>[2x]MTPNWSELVAAADPALVLPSGERRAEVAVPGPLRLDALLDLGEGHAVGVVRSADAARWTVPLVRDGAGGVRRSRPGDGTAEHLVAALARRGATPDAAFVLEAFTGAAPVTGERGIIVDQTNESVIVGECAVVKWAVRLPAEGEPGSPAAQRIAALARGGFTEMPRPWGLLTLAEGAQPVLLASVVAYLPGALDGWDWAVDDVRRLARGEL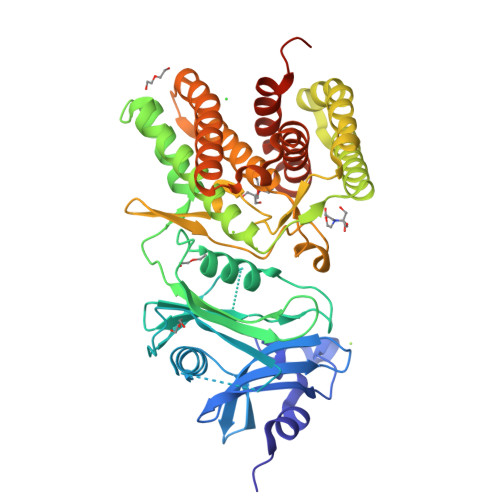TMDQALLPAAQLGTLTARMHAALAARGRTPATAADVAAWGVRMREELDEAVASVPGAEGERLKAWAPRIADVYAELDALAGTPLIDVHGDFHVGQILRADGRYAVVDFDGNPVLPADQRAARQPAALDVVGMTASLDHVGRVVVFRTPDVDPAPVRAWIAAAQRSFLDAYRTTLARLDADDLFDDRLLTPLRYAQEVREYLYAVRHLPHWVYVPDLSLTDLLPERLKDKLAAALEHHHHHH(8M)-8-{3-[(3S)-1-(2-cyclohexylethyl)piperidin-3-yl]-5-oxo-4,5-dihydro-1H-1,2,4-triazol-1-yl}quinolin-2(1H)-one 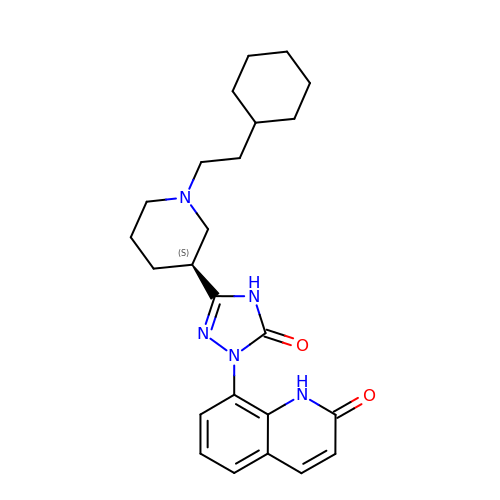| C24 H31 N5 O2 | PKPAUALIHFTDDG-IBGZPJMESA-N> MRGSHHHHHHGSDTMGLFDKLKKLVSDDSASAGAIEIIAPLSGEIVNIEDVPDVVFAEKIVGDGIAIKPTGNKMVAPVNGTIGKIFETNHAFSIESDDGVELFVHFGIDTVELKGEGFTRIAEEGQTVKAGDTVIEFDLALLEEKAKSTLTPVVISNM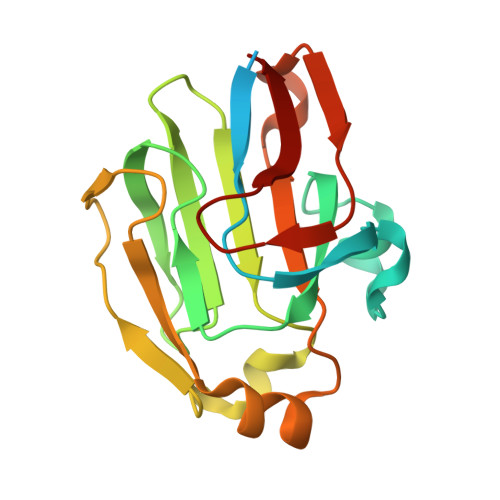DEIKELNKLSGSVVVGETPVLRVTK>[2x]MHHHHHHSSGRENLYFQGHCKVSLLDDTVYECVVEKHAKGQDLLKRVCEHLNLLEEDYFGLAIWDNATSKTWLDSAKEIKKQVRGVPWNFTFNVKFYPPDPAQLTEDITRYYLCLQLRQDIVAGRLPCSFATLALLGSYTIQSELGDYDPELHGVDYV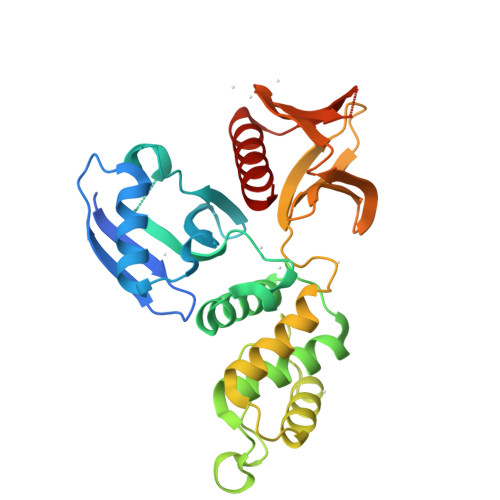SDFKLAPNQTKELEEKVMELHKSYRSMTPAQADLEFLENAKKLSMYGVDLHKAKDLEGVDIILGVCSSGLLVYKDKLRINRFPWPKVLKISYKRSSFFIKIRPGEQEQYESTIGFKLPSYRAAKKLWKVCVEHHTFFR>PGSMDQTYSLESFLNHVQKRDPNQTEFAQAVREVMTTLWPFLEQNPKYRQMSLLERLVEPERVIQFRVVWVDDRNQVQVNRAWRVQFSSAIGPYKGGMRFHPSVNLSILKFLGFEQTFKNALTTLPMGGGKGGSDFDPKGKSEGEVMRFCQALMTELYRHLGADTDVPAGDIGVGGREVGFMAGMMKKLSNNTACVFTGKGLSFGGSLIRPEATGYGLVYFTEAMLKRHGMGFEGMRVSVSGSGNVAQYAIEKAMEFGARVITASDSS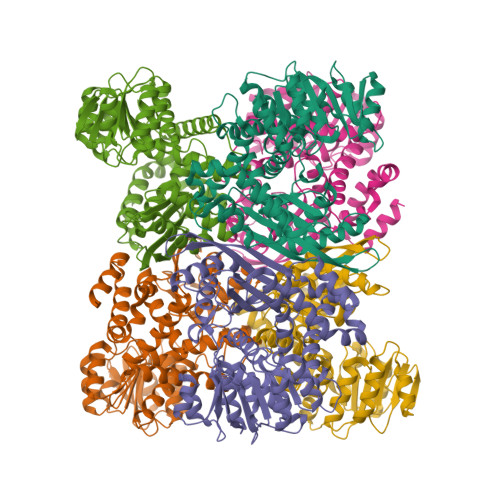GTVVDESGFTKEKLARLIEIKSSRDGRVADYAKEFGLVYLEGQQPWSVPVDIALPCATQNELDVDAAHQLIANGVKAVAEGANMPTTIEATELFQQAGVLFAPGKAANAGGVATSGLEMAQNAARLGWKAEKVDARLHHIMLDIHHACVEHGGEGEQTNYVQGANIAGFVKVADAMLAQGVI[12x]> MKTLTGADALEFHKKLKERNKALHASDLELALVHADAVGKERFDLEELEKICDTSDAGRLTDAKERNDIYERMY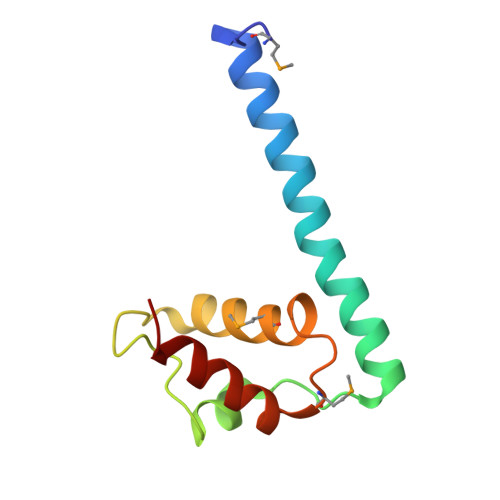YVEYPNVMTLKEFAHIVETLFSWS>KPIEIIGAPFSKGCPRGGVEKGPAALRKAGLVEKLKETEYNVRDHGDLAFVDVPNDSPFQIVKNPRSVGKANEQLAAVVAETQKNGTISVVLGGDHSMAIGSISGHARVHPDLAVIWVDAHTDINTPLTTSSGNLAGQPVAFLLKELKGKFPDVPGFSWVTPAISAKDIVYIGLRDVDPGEHYIIKTLGIKYFSMTEVDKLGIGKVMEETFSYLLGRKKRPIHLSFDVDGLDPVFTPATGTPVVGGLSYREGLYITEEIYKTGLLSGLDIMEVNPTLGKTPEEVTRTVNTAVALTLSAFGTKREGN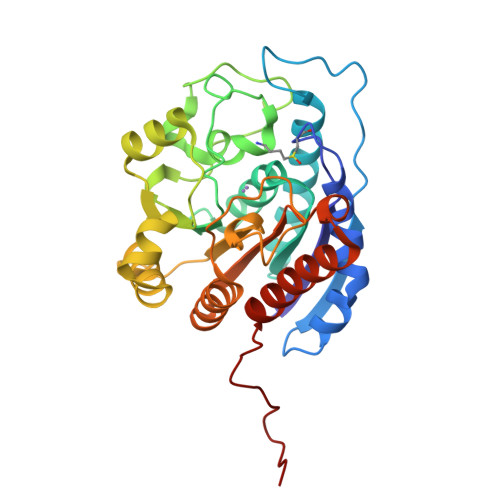HKPETDYL[3x]> MTTAARRPAPTTAGAGWDAGVGALVNPSRR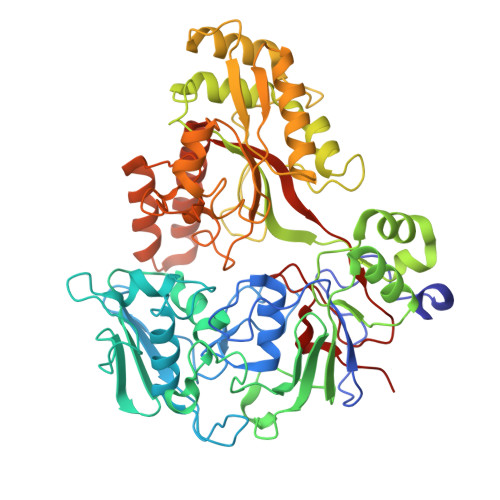RGGTLRLVSSADVDSLDPARTYYVWVWLLQRLLNRTLMAYPTDPGPAGLVPAPDLAEGPGEVSDGGRTWTYRLRRGLRYDDGTPITSDDVRHAVQRVFAQDVLPGGPTYLIPLLDDPERPYPGPYRTDEPLRSVLTPDEHTIVFRLTRPFSDFDHLMAQPCAAPVPRRSDTGADYGRDPRSSGPYRVARHEPDTLLHLERNPHWDRATDPIRPALPDRVELTIGLDVDVLDARLIAGEFDINLEGRGLQHAAQRRATADEVLRSHTDNPRTSFLHFVAMQPHIPPFDNVHVRRAVQYAADKILLQDARGGPVNGGDLTTALFPPTLPAHQDLDLYPTGPDLRGDLDAARAELAAAGLPDGFRAVIGTQRGKFRLVADAVVESLARVGIELTVKELDVATYFSLGAGHPETVREHGLGLLVTDWGADFPTEYGFLAPLVDGRQIKRNGGNWNLPELDDPEVNALIDETLHTTDPAARAELWRAVERRVMEHAVLLPLVHDKTLHFRNPWVTNVYVHPAFGLYDIQAMGLAEED> MGSDRSCVLSVFQTILKLVIFVAIFGAAISSRLFAVIKFESIIHEFDPWFNYRATKYLVNNSFYKFLNWFDDRTWYPLGRVTGGTLYPGLMTTSAFIWHALRNWLGLPIDIRNVCVLFAPLFSGVTAWATYEFTKEIKDASAGLLAAGFIAIVPGYISRSVAGSYDNEAIAITLLMVTFMFWIKAQKTGSIMHATCAALFYFYMVSAWGGYVFITNLIPLHVFLLILMGRYSSKLYSAYTTWYAIGTVASMQIPFVGFLPIRSNDHMAALGVFGLIQIVAFGDFVKGQISTAKFKVIMMVSLFLILVLGVVGLSALTYMGLIAPWTGRFYSLWDTNYAKIHIPIIASVSEHQPVSWPAFFFDTHFLIWLFPAGVFLLFLDLKDEHVFVIAYSVLCSYFAGVMVRLMLTLTPVICVSAAVALSKIFDIYLDFKTSDRKYAIKPAALLAKLIVSGSFIFYLYLFVFHSTWVTRTAYSSPSVVLPSQTPDGKLALIDDFREAYYWLRMNSDEDSKVAAWWDYGYQIGGMADRTTLVDNNTWNNTHIAIVGKAMASPEEKSYEILKEHDVDYVLVIFGGLIGFGGDDINKFLWMIRISEGIWPEEIKERDFYTAEGEYRVDARASETMRNSLLYKMSYKDFPQLFNGGQATDRVRQQMITPLDVPPLDYFDEVFTSENWMVRIYQLKKDDAQGRTLRDVGELTRSSTKTRRSIKRPELGLRV;> MISDEQLNSLAITFGIVMMTLIVIYHAVDSTMSPKNRTLQVDGGSGGSLEVLFQGPTETSQVAPA;> MTYEQLYKEFHSSKSFQPFIHLDTQPKFAICGLIVTLAVLSSALFAVGSKSSYIKKLFFYTILSVIGSLFAGLTTVFASNSFGVYV;> MAKAPKANTPKVTSTSSAVLTDFQETFKTSKRAYFAQIEKYPKLKLIDTFCFFLVLLGVIQCTFIILIRDNFPFNAFLAGFIICVGQFVLLMSLRLQLCNSFPGISKNRAFAEFIVASLILHFVCLHFIN;> MRQVWFSWIVGLFLCFFNVSSAAQYEPPATWENVDYKRTIDVSNAYISETIEITIKNIASEPATEYFTAFESGIFSKVSFFSAYFTNEATFLNSQLLANSTTAPGDDGESEIRYGIIQFPNAISPQEEVSLVIKSFYNTVGIPYPEHVGMSEEQHLLWETNRLPLSAYDTKKASFTLIGSSSFEEYHPPNDESLLGKANGNSFEFGPWEDIPRFSSNETLAIVYSHNAPLNQVVNLRRDIWLSHWASTIQFEEYYELTNKAAKLSKGFSRLELMKQIQTQNMRQTHFVTVLDMLLPEGATDHYFTDLVGLVSTSHAERDHFFIRPRFPIFGGWNYNFTVGWTNKLSDFLHVSSGSDEKFVASIPILNGPPDTVYDNVELSVFLPEGAEIFDIDSPVPFTNVSIETQKSYFDLNKGHVKLTFSYRNLISQVANGQVLIKYDYPKSSFFKKPLSIACYIFTALMGVFVLKTLNMNVTN;> MQFFKTLAALVSCISFVLAYVAQDVHVSFPSTAGKSRVMIGKVEPRIGIDETVPTTITVEDPNEVIQVNFAIESTNKPFQNTLLIGLPNKNLEMAFEPEIKDNGKLSMYKYRIDLAKLDAALLQEASRSPEPIKATLILASSTAKPKENLFREILQLNLNFDVDHSDSSLVDKFGIKPEIHHIFHAEPKRVAKPIAVIFVLIIFITILSLIVTWLNSCAAAFNNIPTGVTAVYFLGFIATIVGFEVIFARYYLGTSIFETLFSSLYLGAPGLLTSTKFLRSFG;> MRTDWNFFFCILLQAIFVVGTQTSRTLVLYDQSTEPLEEYSVYLKDLEQRNYKLEYLDINSTSTTVDLYDKEQRLFDNIIVFPTKGGKNLARQIPVKQLIKFFENEGNILCMSSPGAVPNTIRLFLNELGIYPSPKGHVIRDYFSPSSEELVVSSNHLLNKYVYNARKSEDFVFGESSAALLENREQIVPILNAPRTSFTESKGKCNSWTSGSQGFLVVGFQNLNNARLVWIGSSDFLKNKNQDSNQEFAKE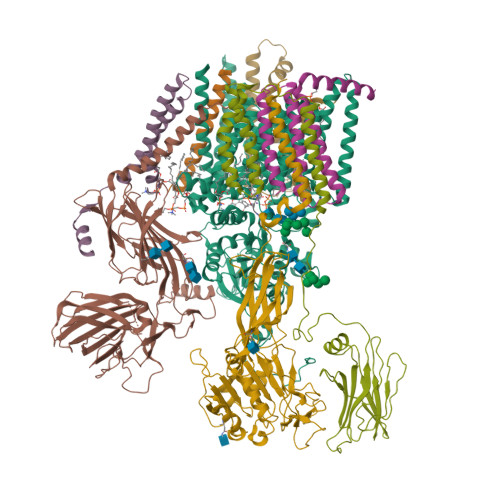LLKWTFNEKSVIKSVHAVHSHADGTSYDEEPYKIKDKVIYSVGFSEWNGEEWLPHIADDIQFELRQVDPYYRLTLSPSGNDSETQYYTTGEFILPDRHGVFTFLTDYRKIGLSFTTDKDVKAIRHLANDEYPRSWEISNSWVYISAICGVIVAWIFFVVSFVTTSSVGKKLETFKKTN;> MNWLFLVSLVFFCGVSTHPALAMSSNRLLKLANKSPKKIIPLKDSSFENILAPPHENAYIVALFTATAPEIGCSLCLELESEYDTIVASWFDDHPDAKSSNSDTSIFFTKVNLEDPSKTIPKAFQFFQLNNVPRLFIFKPNSPSILDHSVISISTDTGSERMKQIIQAIKQFSQVNDFSLHLPMDWTPIITSTIITFITVLLFKKQSKLMFSIISSRIIWATLSTFFIICMISAYMFNQIRNTQLAGVGPKGEVMYFLPNEFQHQFAIETQVMVLIYGTLAALVVVLVKGIQFLRSHLYPETKKAYFIDAILASFCALFIYVFFAALTTVFTIKSPAYPFPLLRLSAPFK;> YAAATSA2-[3,5-bis(fluoranyl)-4-[[3-[5-methoxy-4-[(3-methoxypyridin-4-yl)amino]pyrimidin-2-yl]indazol-1-yl]methyl]phenoxy]ethanol | C27 H24 F2 N6 O4 | 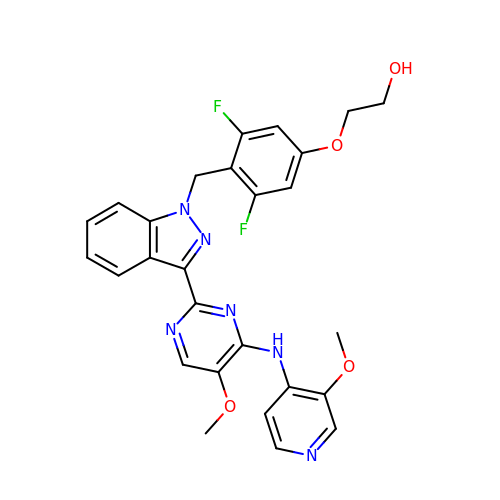QVOGVAVHOLLLAZ-UHFFFAOYSA-N>[2x]EQARPADDALAALGAQLFVDPALSRNATQSCATCHDPARAFTDPREGKAGLAVSVGDDGQSHGDRNTPTLGYAALVPAFHRDANGKYKGGQFWDGRADDLKQQAGQPMLNPVEMAMPDRAAVAARLRDDPAYRTGFEALFGKGVLDDPERAFDAAAEALAAYQATGEFSPFDSKYDRVMRGEEKFTPLEEFGYTVFITKNCRLCHMQ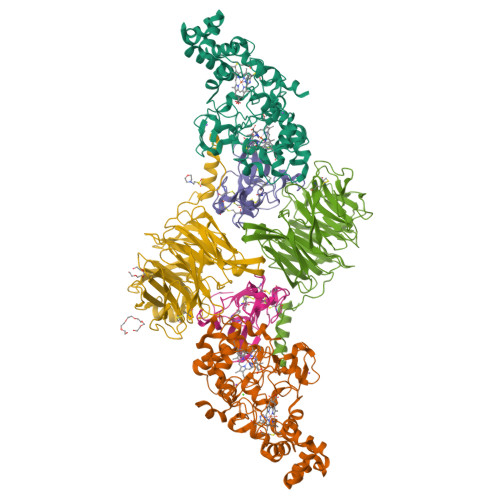RKQGVAERETFTNFEYHNIGLPVNETAREASGLGADHVDHGLLARPGIEDPAQSGRFKVPSLRNVAVTGPYMHNGVFTDLRTAILFYNKYTSRRPEAKINPETGAPWGEPEVARNLSLAELQSGLMLDDGRVDALVAFLETLTDRRYEPLLEESRAAQKDHHHHHH;>[2x]ADAPAGTDPRAKWVPQDNDIQACDYWRHCSIDGNICDCSGGSLTNCPPGTKLATASWVASCYNPTDGQSYLIAYRDCCGYNVSGRCPCLNTEGELPVYRPEFANDIIWCFGAEDDAMTYHCTISPIVGKASHHHHHH;>[2x]QDAPEAETQAQETQGQAAARAAAADLAAGQDDEPRILEAPAPDARRVYVNDPAHFAAVTQQFVIDGEAGRVIGMIDGGFLPNPVVADDGSFIAHASTVFSRIARGERTDYVEVFDPVTLLPTADIELPDAPRFLVGTYPWMTSLTPDGKTLLFYQFSPAPAVGVVDLEGKAFKRMLDVPDCYHIFPTAPDTFFMHCRDGSLAKVAFGTEGTPEITHTEVFHPEDEFLINHPAYSQKAGRLVWPTYTGKIHQIDLSSGDAKFLPAVEALTEAERADGWRPGGWQQVAYHRALDRIYLLVDQRDEWRHKTASRFVVVLDAKTGERLAKFEMGHEIDSINVSQDEKPLLYALSTGDKTLYIHDAESGEELRSVNQLGHGPQVITTADMG>[3x]EFSPAAAPPTLPPYFMKGSMIQLANGELKKVEDLKTEDFIQSAEMSNDLKIDSSTVERIEDSHSPGVAVIQFAVGEHRAQVSVEVLVEYPFFVFGQGWSSCCPERTSQ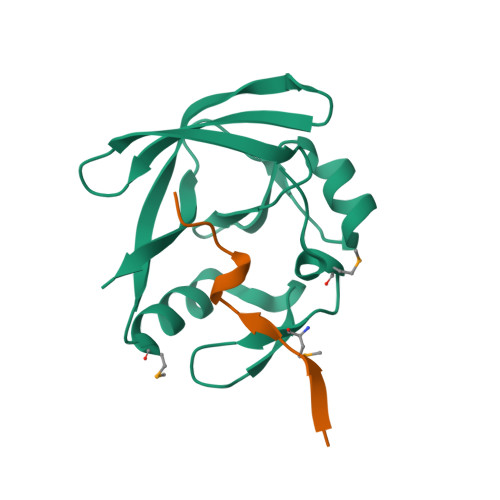LFDLPCSKLSVGDVCISLTLK;>EPRSVAVFPWHSLVPFLAPSQ[3x]>GPLGSMATSRYEPVAEIGVGAYGTVYKARDPHSGHFVALKSVRVPNGGGGGGGLPISTVREVALLRRLEAFEHPNVVRLMDVCATSRTDREIKVTLVFEHVDQDLRTYLDKAPPPGLPAETIKDLMRQFLRGLDFLHANCIVHRDLKPENILVTSGGTVKLADFGLARIYSYQMALTPVVVTLWYRAPEVLLQSTYATPVDMWSVGCIFAEMFRRKPLFCGNSEADQLGKIFDLIGLPPEDDWPRDVSLPRGAFPPRGPRPVQSVVPEMEESGAQLLLEMLTFNPHKRISAFRALQHSYLHKDEGNPE[2x];>[2x]MDYKDDDDKSPGGSMELLCCEGTRHAPRAGPDPRLLGDQRVLQSLLRLEERYVPRASYFQCVQREIKPHMRKMLAYWMLEVCEEQRCEEEVFPLAMNYLDRYLSCVPTRKAQLQLLGAVCMLLASKLRETTPLTIEKLCIYTDHAVSPRQLRDWEVLVLGKLKWDLAAVIAHDFLAFILHRLS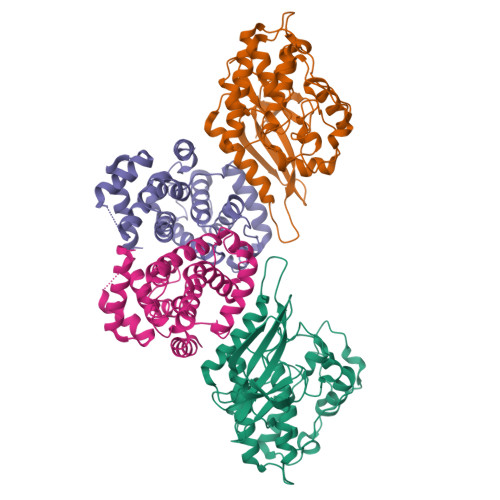LPRDRQALVKKHAQTFLALCATDYTFAMYPPSMIATGSIGAAVQGLGACSMSGDELTELLAGITGTEVDCLRACQEQIEAALRESLREAAQTSSSPAPKAPRGSSSQGPSQTSTPTDVTAIHL>MTERIRNVALRSKVCPAETASELIKHGDVVGTSGFTGAGYPKEVPKALAQRMEAAHDRGEKYQISLITGAATGPQLDGELAKANGVYFRSPFNTDATMRNRINAGETEYFDNHLGQVAGRAVQGNYGKFNIALVEATAITEDGGIVPTSSVGNSQTFLNLAEKVIIEVNEWQNPMLEGIHDIWDGNVSGVPTRDIVPIVRADQRVGGPVLRVNPDKIAAIVRTNDRDRNAPFAAPDETAKAIAGYLLDFFGHEVKQNRLPPSLLPLQSGVGNVANAVLEGLKEGPFENLVGYSEVIQDGMLAMLDSGRMRIASASSFSLSPEAAEEINNRMDFFRSKIILRQQDVSNSPGIIRRLGCIAMNGMIEADIYGNVNSTRVMGSKMMNGIGGSGDFARSSYLSIFLSPSTAKGGKISAIVPMAAHVDHIMQDAQIFVTEQGLADLRGLSPVQRAREIISKCAHPDYRPMLQDYFDRALKNSFGK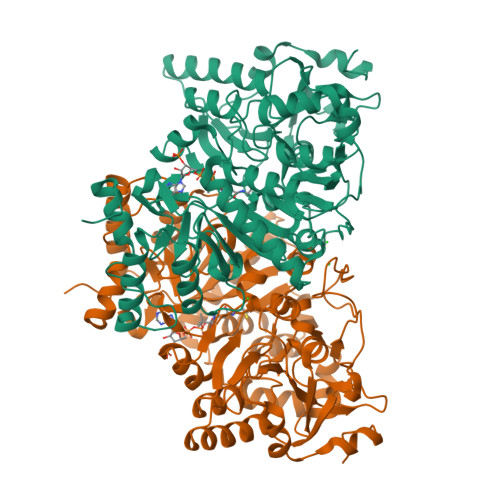HTPHLLTEALSWHQRFIDTGTMLPSSLEHHHHHH[2x]> MIDVIMTGELLKTVTRAIVALVSEARIHFLEKGLHSRAVDPANVAMVIVDIPKDSFEVYNIDEEKTIGVDMDRIFDISKSISTKDLVELIVEDESTLKVKFGSVEYKVALIDPSAIRKEPRIPELELPAKIVMDAGEFKKAIAAADKISDQVIFRSDKEGFRIEAKGDVDSIVFHMTETELIEFNGGEARSMFSVDYLKEFCKVAGSGDLLTIHLGTN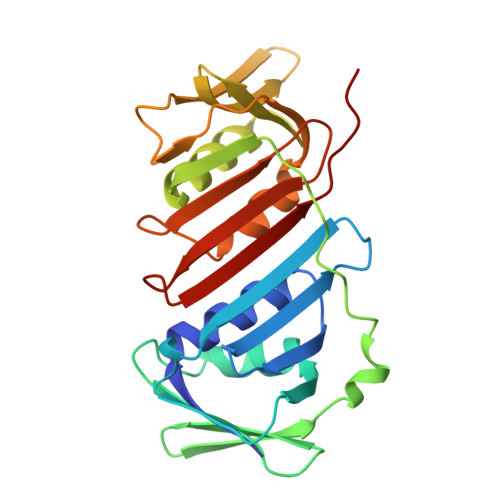YPVRLVFELVGGRAKVEYILAPRIESE> FKDPNAPKRPPSAFFLFCSEYRPKIKGEHPGLSIGDVAKKLGEMWNNTAADDKQPYEKK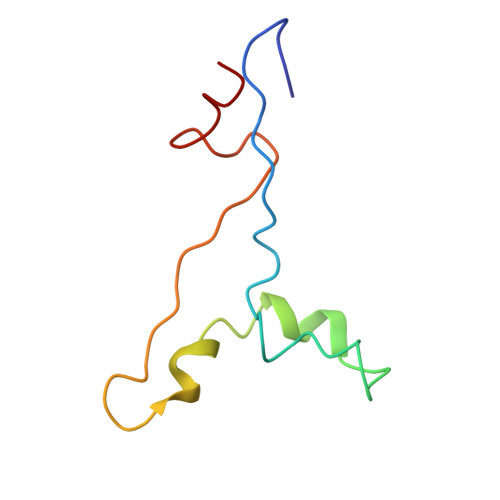AAKLKEKYEKDIAAYR3-[5-[3,5-bis(chloranyl)phenyl]-4-phenyl-1,3-oxazol-2-yl]propanoic 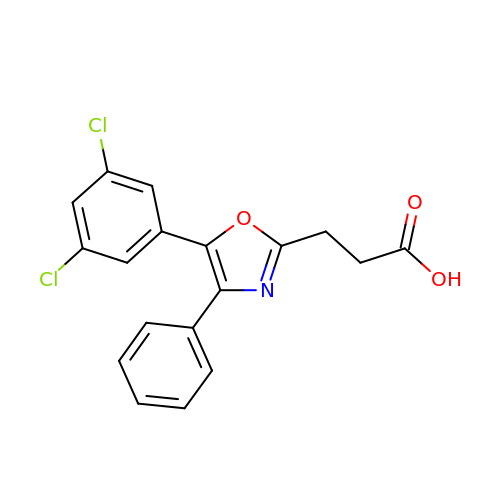acid | C18 H13 Cl2 N O3 | MNBKLGOJIXFSTI-UHFFFAOYSA-N Forkhead box (FOX) proteins belong to an evolutionarily conserved family of transcription factors expressed from yeast to humans, and possess a highly conserved DNA-binding domain (DBD), called the ‘forkhead box’ domain. Most FOX proteins bind to the typical FOX DNA-binding element (FBE) 5′-RYAAAYA-3′ (R = A or G, Y = C or T) to regulate the transcription of their target genes. Here, we found that FOX family proteins bind to the non-canonical homotypic cluster of the p53 promoter region (TP53). Analysis of crystal structures of FOX proteins (FOXL2 and FOXA1) bound to the p53 homotypic cluster indicated that they interact with a 2:1 stoichiometry accommodated by FOX-induced DNA allostery.

We further determined the co-crystal structure of FOXA1-DBD in complex with p53-DNA (5′-AAATATTTATTATCGA-3′). The crystals of the FOXA1-DBD complex with p53-DNA also showed 2:1 stoichiometry, and FOXA1-DBD1 bound to the major groove of the FBE1 site through helix 3 of FOXA1-DBD, which is similar to FOXL2-DBD. However, FOXA1-DBD2 bound to DNA at an unexpected position distinct from FOXL2, where helix 3 of FOXA1-DBD2 bound to the major groove of extended DNA formed by crystal packing, and formed apparent protein–protein dimerization with FOXA1-DBD1. In FOXA1-DBD1, His220 (corresponding to His104 in FOXL2) made contact with the base of T8′ and also with that of A10 via a water molecule (3.0–3.3 Å). Asn216 (Asn100 in FOXL2) formed bidentate hydrogen bonds with the base of A10′ (2.9–3.1 Å). In the wing 1 region, the backbone of Ser242 and that of A5 formed a hydrogen bond, and the side chain of Lys240 was directed to the major groove of DNA, interacting with the bases of A2 and A3, and water-mediated interaction with T16′ (3.3 Å), constituting additional contacts between FOXA1 and p53-DNA. Distinct from FOXL2, the protein dimer interface between the N- and C-termini of FOXA1-DBD1 and FOXA1-DBD2 was observed in the structure of FOXA1-DBD in complex with p53-DNA. Tyr173 interacted with Gln184 in neighboring FOXA1-DBD molecules. Importantly, Ser174 and Ser177 in FOXA1-DBD1 and FOXA1-DBD2 formed Mg2+ coordination with their backbone and side chains. The converged dimerization, which refers to the opposite direction of FOXA1-DBD molecules on DNA, was observed, involving unexpected interaction between N-terminal parts of each protein, which was mediated by magnesium ions.

>GAMGSHAKPPYSYISLITMAIQQAPSKMLTLSEIYQWIMDLFPYYRQNQQRWQNSIRHSLSFNDCFVKVARSPDKPGKGSYWTLHPDSGNMFENGCYLRRQK[4x]> MAATDIARQVGEGCRTVPLAGHVGFDSLPDQLVNKSVS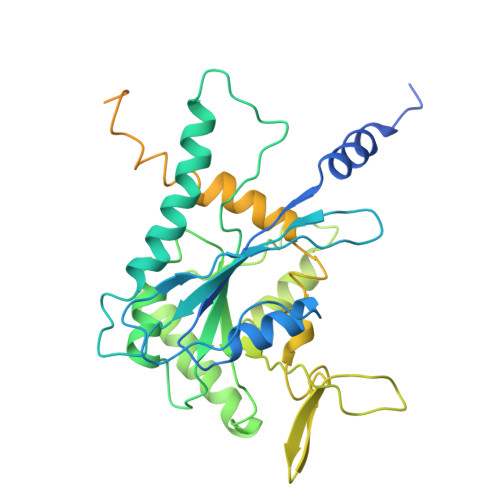QGFCFNILCVGETGLGKSTLMDTLFNTKFEGEPATHTQPGVQLQSNTYDLQESNVRLKLTIVSTVGFGDQINKEDSYKPIVEFIDAQFEAYLQEELKIRRVLHTYHDSRIHVCLYFIAPTGHSLKSLDLVTMKKLDSKVNIIPIIAKADAISKSELTKFKIKITSELVSNGVQIYQFPTDDESVAEINGTMNAHLPFAVIGSTEELKIGNKMMRARQYPWGTVQVENEAHCDFVKLREMLIRVNMEDLREQTHTRHYELYRRCKLEEMGFKDTDPDSKPFSLQETYEAKRNEFLGELQKKEEEMRQMFVQRVKEKEAELKEAEKELHEKFDRLKKLHQDEKKKLEDKKKSLDDEVNAFKQRKTAAELLQSQGSQAGGSQTLKRDKEKKN4-[(4-methylpiperazin-1-yl)methyl]-N-(4-methyl-3-{[1-(pyridin-3-ylcarbonyl)piperidin-4-yl]oxy}phenyl)-3-(trifluoromethyl)benzamide | C32 H36 F3 N5 O3 | 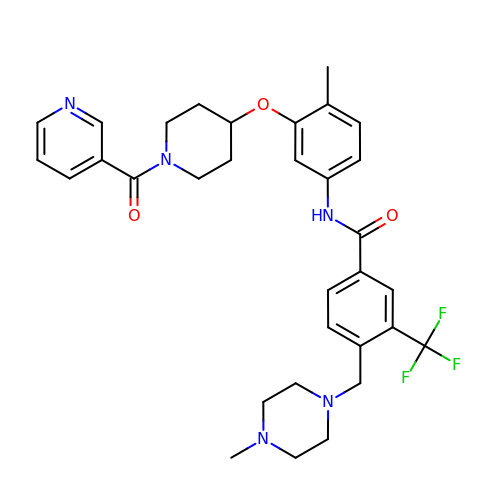CBLZTDLZCXMNCE-UHFFFAOYSA-N> EDSLTKQPEEVFDVLEKLGEGSYGSVFKAIHKESGQVVAIKQVPVESDLQEIIKEISIMQQCDSPYVVKYYGSYFKNTDLWIVMEYCGAGSVSDIIRLRNKTLIEDEIATILKSTLKGLEYLHFMRKIHRNIKAGNILLNTEGHAKLADFGVAGQLTDTMAKRNTVIGTPFWMAPEVIQEIGYNCVADIWSLGITSIEMAEGKPPYADIHPMRAIFMIPTNPPPTFRKPELWSDDFTDFVKK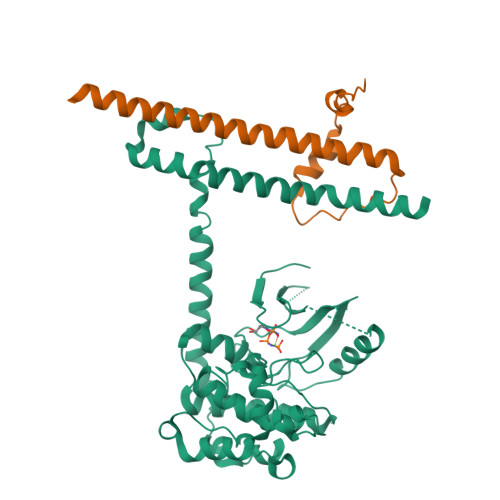CLVKNPEQRATATQLLQHPFIKNAKPVSILRDLITEAMEIKAKRHEEQQRELEEEENWKVPQDGDFDFLKNLSLEELQMRLKALDPMMEREIEELRQRYTAKRQPILDAMDAKKRRQQNF;> SLLVPANPYHTAEIPDWLQVYARAPVKYDHILKWELFQLADLDTYQGMLKLLFMKELEQIVKMYEAYRQALLTELENRKQRQQWYAQQHGKNF>AADIVQMVEDLTGKLTALAWALFLLSWSIGWTLRGSPIPSSRIKRVGNSLIEDSMWAALWLALGTTVFAVIVRLAGIVNEVLLG[30x]

Here, we determine atomic structures by cryo-electron microscopy of three conjugative pili, two from hyperthermophilic archaea (Aeropyrum pernix and Pyrobaculum calidifontis) and one encoded by the Ti plasmid of the bacterium Agrobacterium tumefaciens, and show that the archaeal pili are homologous to bacterial mating pili. With structures for four bacterial conjugation pili (pED208, F, pKpQIL, and pTiC58 from A. tumefaciens) and two archaeal ones (A. pernix and P. calidifontis), it is clear that there is a common architecture for all and obvious homology, despite negligible sequence similarity. Each prokaryotic pilin subunit consists of two or three hydrophobic α-helices, with kinks appearing in some of the helices, such as in A. pernix and A. tumefaciens. Hence, pore diameters of all prokaryotic conjugative pili are sufficiently wide for the passage of ssDNA, but not dsDNA.

Here, using cryo-electron microscopy (cryo-EM), we show that a protein from the hyperthermophilic archaeon Aeropyrum pernix, a homolog of CedA1, forms a pilus which is structurally homologous to bacterial conjugative pili. The reconstruction of this pilus to 3.3 Å resolution allowed us to determine the pilin identity directly from the cryo-EM map. While in the A. pernix filament the helical rise and twist per subunit were 3.6 Å and 76.5°, respectively, in the P. calidifontis filament these parameters were 5.0 Å and 74.2°. In A. pernix, there are two lipids in every ASU, one of which adopts a partially folded conformation, with one of the isoprenoid chains folding back on itself, while the other has a crescent-like shape. Instead, an unusual C25, C25-diether with a phospho-dihexose head group was the main lipid species observed by mass spectrometry of a cellular membrane preparation of A. pernix, consistent with the previous identification of this lipid in A. pernix. Both non-protein densities in the A. pernix map could be fit with this lipid, suggesting that the same lipid is present in two different conformations. The contacts with helix α1 are mediated by leucine-rich hydrophobic interactions and one charged interaction between the phosphate head group and the positively charged Lys15. In total, each CedA1 subunit will make contacts with 10 lipid molecules. In A. pernix each pilin is bound to two diether lipids with phosphorylated dihexose (i.e., glucose-inositol) head groups. One of these lipids faces the lumen of the central channel where it might also provide a similar negative charge to facilitate DNA transfer.> SNAD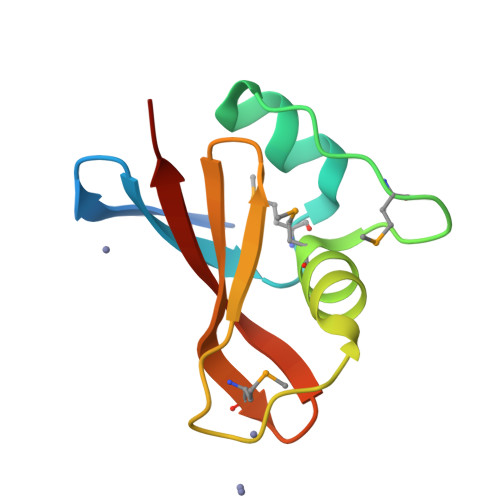EVENLYTQVADNEYLVQGRMLIDEFNEVFETDLHMSDVDTMAGYLITALGTIPDEGEKPSFEVGNIKLTAEEMEGTRLLVLRVHFYDEE>GAMGSKFSVEEYLVHAL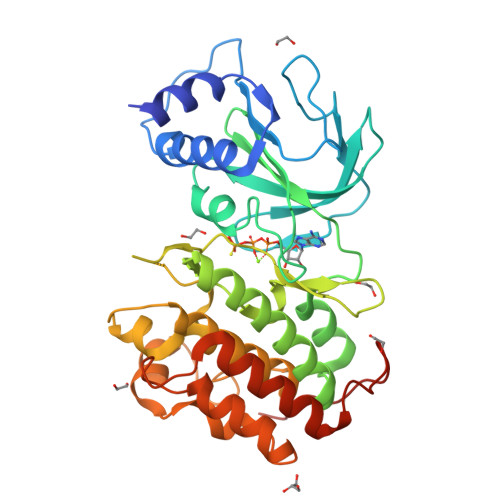QGSVSSGQAHSLTSLAKTWAARGSRSREPSPKTEDNEGVLLTEKLKPVDYEYREEVHWATHQLRLGRGSFGEVHRMEDKQTGFQCAVKKVRLEVFRAEELMACAGLTSPRIVPLYGAVREGPWVNIFMELLEGGSLGQLVKEQGCLPEDRALYYLGQALEGLEYLHSRRILHGDVKADNVLLSSDGSHAALCDFGHAVCLQPDGLGKDLLTGDYIPGTETHMAPEVVLGRSCDAKVDVWSSCCMMLHMLNGCHPWTQFFRGPLCLKIASEPPPVREIPPSCAPLTAQAIQEGLRKEPIHRVSAAELGGKVNRALQQVGGLKSPWRGEYKEPRHPPPNQA[2x]> XFF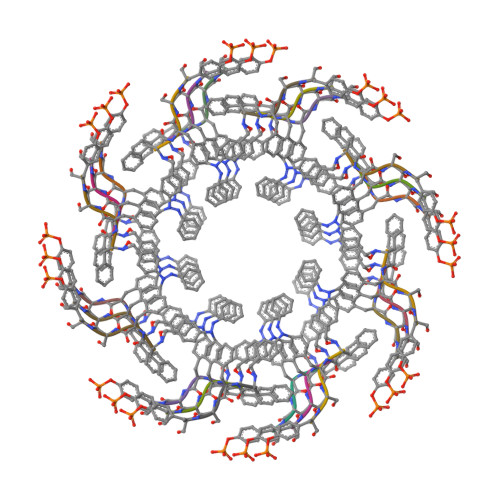SW>[2x]MITQEMKDLINNQLAMVATVDAKGQPNIGPKRSMRLWDDKTFIYNENTDGQTRINIEDNGKIEIAFVDRERLLGYRFVGTAEIQTEGAYYEAAKKWAQGRMG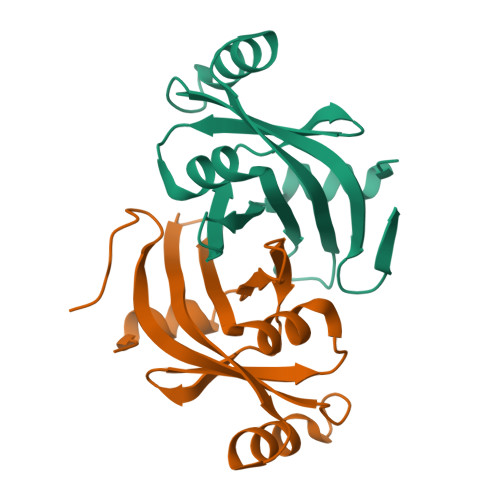VPKAVGIIHVERIFNLQSGANAGKEINSESNKGELNSKLEGKPIPNPLLGLDSTRTGHHHHHH> SNAMQAIRSILVVIEPDQLEGLALKRAQLIAGVTQSHLHLLVCEKRRDHSAALNDLAQELREEGYSVSTNQAWKDSLHQTIIAEQQAEGCGLIIKQHFPDNPLKKAILTPDDWKLLRFAPCPVLMTKTARPWTGGKILAAVDVGNNDGEHRSLHAGIISHAYDIAGLAKATLHVISAHPSPMLSSADPTFQL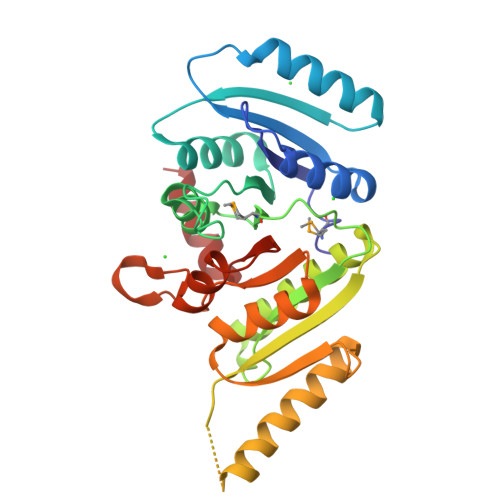SETIEARYREACRTFQAEYGFSDEQLHIEEGPADVLIPRTAQKLDAVVTVIGTVARTGLSGALIGNTAEVVLDTLESDVLVLKPDDIIAHLEELASK> MQNAESWFKKYWHLSVLVIAALISVKLRILNPWNSVFTWTVRLGGNDPWYYYRL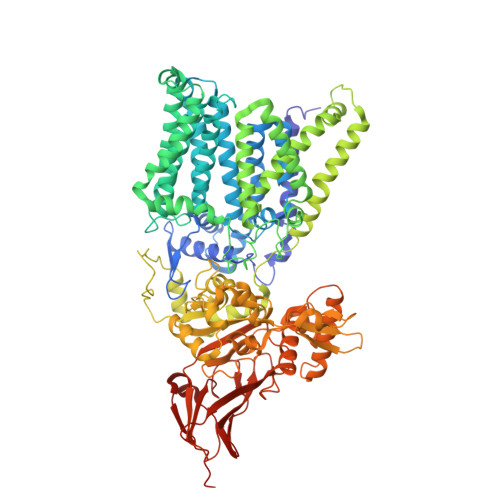IENTIHNFPHRIWFDPFTYYPYGSYTHFGPFLVYLGSIAGIIFSATSGESLRAVLAFIPAIGGVLAILPVYLLTREVFDKRAAVIAAFLIAIVPGQFLQRSILGFNDHHIWEAFWQVSALGTFLLAYNRWKGHDLSHNLTARQMAYPVIAGITIGLYVLSWGAGFIIAPIILAFMFFAFVLAGFVNADRKNLSLVAVVTFAVSALIYLPFAFNYPGFSTIFYSPFQLLVLLGSAVIAAAFYQIEKWNDVGFFERVGLGRKGMPLAVIVLTALIMGLFFVISPDFARNLLSVVRVVQPKGGALTIAEVYPFFFTHNGEFTLTNAVLHFGALFFFGMAGILYSAYRFLKRRSFPEMALLIWAIAMFIALWGQNRFAYYFAAVSAVYSALALSVVFDKLHLYRALENAIGARNKLSYFRVAFALLIALAAIYPTYILADAQSSYAGGPNKQWYDALTWMRENTPDGEKYDEYYLQLYPTPQSNKEPFSYPFETYGVISWWDYGHWIEAVAHRMPIANPFQAGIGNKYNNVPGASSFFTAENESYAEFVAEKLNVKYVVSDIEMETCKYYAMAVWAEGDLPLAEKYYGGYFYYSPTGTFGYANSQWDIPLNSIIIPLRIPSELYYSTMEAKLHLFDGSGLSHYRMIYESDYPAEWKSYSSQVNLNNESQVLQTALYEAVMRARYGVSPTMGTQEVLYKYAYTQLYEKKMGIPVKIAPSGYVKIFERVKGAVVTGKVSANVTEVSVNATIKTNQNRTFEYWQTVEVKNGTYTVVLPYSHNSDYPVKPITPYHIKAGNVVKEITIYESQVQNGEIIQLDLELALVPR> SNAMFAPQGLAQFIKVNVTLENGEPVFIYTDANGQVCQGDITVTQAGTITYLLNDQTLKGLKFVGVGFVTPFDGIIDAVTISSDGMLVQLVDLDKTPGT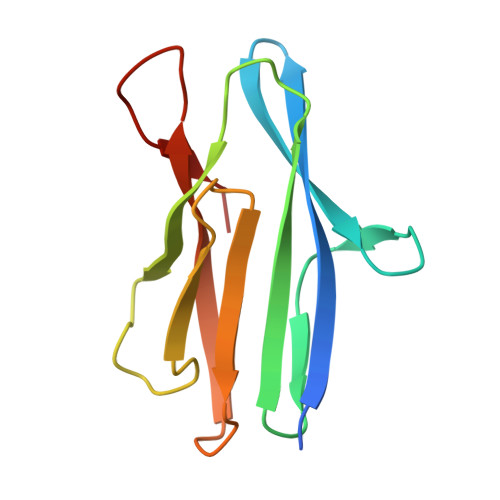TAFQFVLSNTANTLLVLSPD> RSMSEVITITKRNGAFQNSSNLSYNNTGISDDENDEEDIYMHDVNSASKSESDSQIVTPGELVTDDPIWMRGHGTYFLDNMTYSSVAGTVSRVNRLLSVIPLKGRYA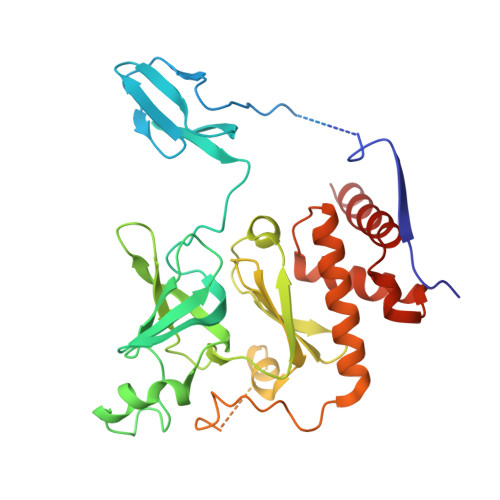PETGDHVVGRIAEVGNKRWKVDIGGKQHAVLMLGSVNLPGGILRRKSESDELQMRSFLKEGDLLNAEVQSLFQDGSASLHTRSLKYGKLRNGMFCQVPSSLIVRAKNHTHNLPGNITVVLGVNGYIWLRKTSQMDLARDTPSANNSSSIKSTGPTGAVSLNPSITRLEEESSWQIYSDENDPSISNNIRQAICRYANVIKALAFCEIGITQQRIVSAYEASMVYSNVGELIEKNVMESIGSDILTAEKMRGNGN GuaB catalyzes the oxidation of the substrate inosine-5´-monophosphate (IMP) to xanthosine 5´-monophosphate (XMP) using NAD+ as a cofactor, and guanosine 5´-monophosphate (GMP) synthase converts XMP to guanosine 5'- monophosphate (GMP) to generate guanine nucleotides essential for cell growth and viability. Indeed, genetic studies have shown that de novo guanine biosynthesis is essential for growth and viability of bacteria both in vitro and in vivo (10–23). Here, we present the first high resolution co-crystal structures of A. baumannii, S. aureus, and E. coli GuaB proteins (cystathionine beta-synthase (CBS) domains deleted), each determined with a matched set of three different inhibitors bound. Similarly, the NAD+ binding region, also where our compounds bind, occurs at the junction between neighboring molecules with side chains from both protomers contributing to ligand binding interactions.

The A. baumannii protein consistently crystallized in space group P21 with eight copies in the asu, forming an octamer composed of two inverted tetramers, relatively rotated to interdigitate the labile “finger” loops (residues 371–381) that mediate much of the tetramer:tetramer interface. We observed a tight overlay of structures across the bacterial strains, highlighting common critical interactions required for potency. These inhibitors mimic the NADH/IMP cofactor interactions by forming strong π-π stacking interactions with IMP while also hydrogen bonding with the conserved glycine (Gly299Ab/302Sa/300Ec) which is one of the two hydrogen bond interactions observed with the NADH amide. The ligand linker segment induces a 90° bend, directing either the amide N-H of G2 and G1 or the imidazole of G8 to form an important hydrogen bond to the conserved glutamic acid (Glu416Ab/417Sa/415Ec) while directing the aryl tail group into a hydrophobic shelf region. This Glu residue underpins species selectivity, because the human homologs (IMPDH1/2) contain a Gln residue at this position that effectively prevents binding. Differences in the polarity of a particular key selectivity residue specifically (Ser250 in E. coli versus Ala252 in S. aureus and Ala249 in A. baumannii) was found to be critical for inhibitor interaction with GuaB which corroborates the observations of previous reports. Enzymatic mechanism of inhibition studies showed GuaBi binds to A. baumannii GuaB uncompetitively with respect to IMP, and via a mixed non-competitive binding type with respect to NAD+. G1 was designed specifically to remove the hydroxy-alcohol that is a substrate of extra-hepatic alcohol-dehydrogenase metabolism, and retained excellent biochemical and in vivo potency. G2 was bactericidal against A. baumannii at 5× Fu/MIC, and G1 was bactericidal above 2× Fu/MIC.

>[8x]MHHHHHHGENLYFQGSMLTIVQEALTFDDVLLLPAYSTVLPKDVSLKTRLTRGIYLNIPLVSAAMDTVTESRMAIAMAQNGGIGILHKNMDIAAQAAEVRRVKKFEAGKAESYPNSCKDDLGRLRVGAAVGTGADTPSRVEALVEAGVDVIVVDTAHGHSAGVIERVRWVKQNFPQVQVIGGNIATGDAALALLDAGADAVKVGIGPGSICTTRIVAGIGMPQISAIDSVASALKDQIPLIADGGIRFSGDMAKAIGAGASTIMVGSLLAGTEEAPGEVEFFQGRYYKAYRGMGSLGAMAGATGSADRYFQDSKAGAEKLVPEGIEGRVPYKGPMGNIVHQMMGGLRSSMGYTGSAVIEDLRQNAKFVKITSAGMSESHVHDVTITKEAPNYRVG> MAKKVKVITDPEVIKVMLEDTRRKILKLLRNKEMTISQLSEILGKTPQTIYHHIEKLKEAGLVEVKRTEMKGNLVEKYYGRTADVFYINLYLGDEELRYIARSRLKTKIDIFKRLGYQFEENELLNIMDRMSQKEFDATVRISKYIEEKEDALKDFSNEDIIHAIEWLSTA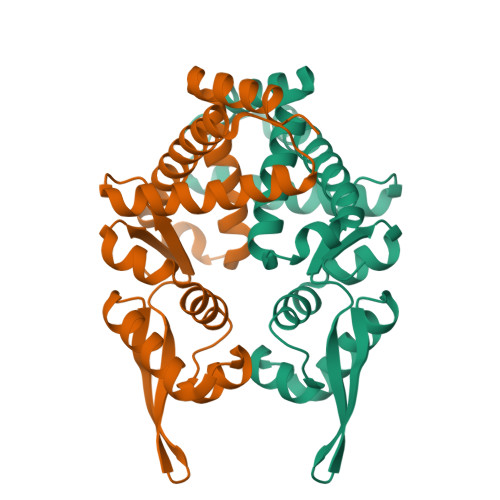ELARDEEYLELLKRLGSILKR> AMREPFKYVDGILYLQAWKELGNITAGFTTKDGGISTGSFHAMNLGLHVNDIVENVHENRRILANKLQKPLENWICSEQVHAHHVEKVGQQEKGSGVYSYEDGISKTDGIYTSNEDVLLTSCYADCVPLYFYAPSHGMIGLAHAGWKGTVQEIA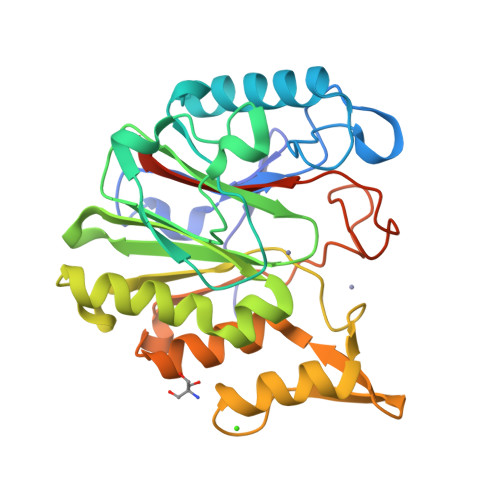KEMIQKWNAEGISSDEIHVAIGPSIGSCCYVVDDRVLTAAQEVVSGAVPHQKISDGQYAINLKEINRILCVQAGIKEEHIVMSSLCTSCEEQLFFSHRRDQGKTGRMLSFIGFKEEGSKLEHHHHHH> GSWKKVQCTLCKSKKH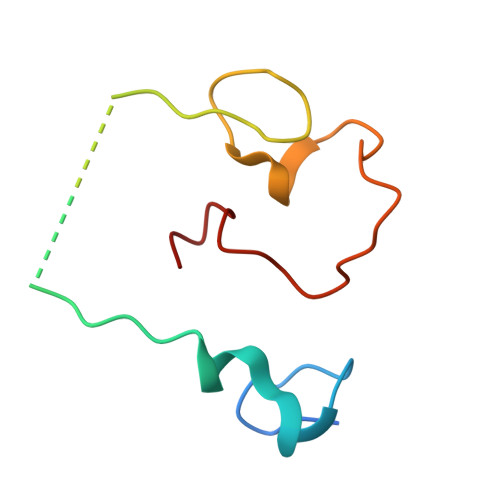SKERCPSIWRAYILVDDNEKAKPKVLPFHTIYCYNCGGKGHFGDDCKEKRSSRVPNEDGSAFTGSNL>SMSKNNIFNKYPTIIHGEARGENDEFVVHTRYPRFLARKSFDDNFTGEMPAKPVNGELGQIGEPRRLAYDSRLGLWLSDFIMLDNNKPKNMEDWLGQLKAACDRIAADDLMLNEDAADLEGWDD[2x];> SMAAFKPNSINYILGLDIGIASVGWAMVEIDEEENPIRLIDLGVRVFERAEVPKTGDSLAMARRLARSVRRLTRRRAH

In this work, we investigate the mechanism of activity of anti-CRISPR protein AcrIIC2Nme. This 123-residue protein was previously shown to inhibit the activity of Neisseria meningitidis CRISPR-Cas9 in vivo and in vitro. We show that AcrIIC2Nme functions by inhibiting loading of the guide RNA molecule, thereby preventing formation of the active CRISPR-Cas9 surveillance complex. We found that it blocks Cas9 binding to sgRNA, thereby inhibiting biogenesis of the surveillance complex. This interference is mediated through an interaction with the arginine-rich bridge helix, which connects the REC lobe to the NUC lobe.

Analysis of the AcrIIC2-Nme1Cas9 crystal by SDS-PAGE revealed that the rest of Nme1Cas9 was digested during crystallization. To confirm this finding, we treated the AcrIIC2-Nme1Cas9 complex with α-chymotrypsin protease, and then crystalized the digested complex. We solved this structure to a resolution of 2.3 Å and found that it was similar to the structure discussed above. The AcrIIC2Nme monomers form a dimer with a negatively charged surface on one side into which the arginine-rich bridge helix nestles. Four residues from each of the AcrIIC2Nme monomers, E17, E24, D108, and N112, make interactions with the bridge helix. In AcrIIC2.1, the side-chain of E17 hydrogen bonds with Nme1Cas9 residues R69 and R73, E24 interacts with residues R73 and R74, while D108 and N112 form hydrogen bonds with the side-chain of R74. Similarly, the side-chains of E24, D108, E17, and N112 of AcrIIC2.2 interact with Nme1Cas9 residues R62, R66, R69, and R70. To further establish the impact of AcrIIC2Nme binding on the assembly of Nme1Cas9 with sgRNA, we compared the structure of AcrIIC2Nme bound to Nme1Cas9 with the Nme1Cas9-sgRNA binary complex by aligning the bridge helix regions. The structural superposition shows that two AcrIIC2Nme monomers make major clashes with stem loops 1 and 2, and slightly overlap the seed region of the sgRNA.>MMKPEDVIKEQCARAKVVAELWHGFTGGAPKAALENLVVEFNKAQQGRCVRPVPQGGYRDLSTKIKAAFAAGKVPTMAQAAENNIALYLEAKALLPIESLGVKLQGVNLTFLNAVRFGGVVYGVPFNKSIQVLYYNKDLLKKHGVPVPATLEEFVAAAKKLSRAEGGPVYWFQPDASTFAYFFFNLGGSYLKDGKLVLNSKEAVEALTLLQNGVKEGWAKPITSGYINQNLGSGPYAFSVDTSAGYTYYLRAAKFDLGVATLPGRTKGQPGYGLVQGTNLVVFRQASKEEQAVAKDFLEFVLSPRAQAVFATATGYVPVTEGALKDPVYQAYAAENPDYATIVRQSRYAKFEPALAEWEQIRFDILGQAIKEAILNKADPKAALD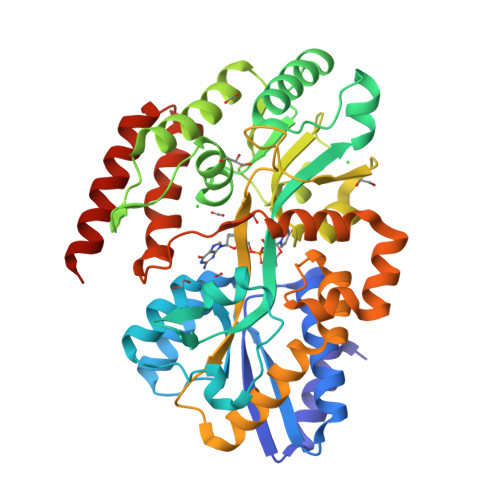RAQKLAEDLLSSRTRHHHHHH[2x]(3~{R})-3-(4-chlorophenyl)-2-[(4-ethynylphenyl)methyl]-3-[[1-(hydroxymethyl)cyclopropyl]methoxy]-6-(2-oxidanylpropan-2-yl)isoindol-1-one | C31 H30 Cl N O4 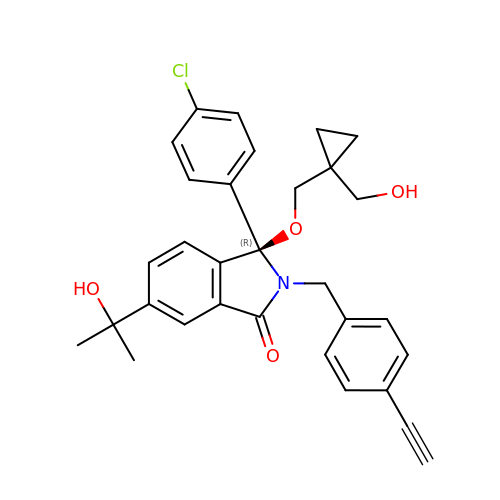| LTEBUYNLVXWZOS-WJOKGBTCSA-N> SNALAFSDMNTGAGKIENGKKALKIVVVGDGAVGKTCLLLAFSKGEIPTAYVPTVFENFSHVMKYKNEEFILHLWDTAGQEEYDRLRPLSYADSDVVLLCFAVNNRTSFDNISTKWEPEIKHYIDTAKTVLVGLKVDLRKDGSDDVTKQEGDDLCQKLGCVAYIEASSVAKIGLNEVFEKSVD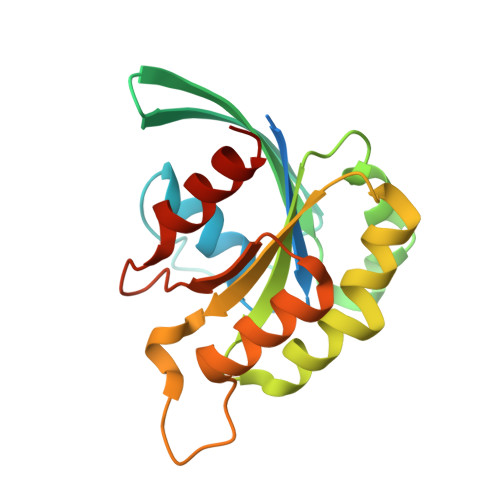CIFSN>[3x]MTPE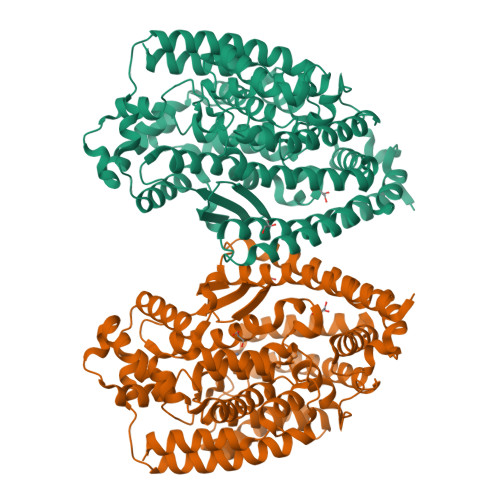AAYQNLLEFQRETAYLASLGALAAWDQRTMIPKKGHEHRARQMAALARLLHQRMTDPRIGEWLEKVEGSPLVQDPLSDAAVNVREWRQAYERARAIPERLAVELAQAESEAESFWEEARPRDDWRGFLPYLKRVYALTKEKAEVLFALPPAPGDPPYGELYDALLDGYEPGMRARELLPLFAELKEGLKGLLDRILGSGKRPDTSILHRPYPVEAQRRFALELLSACGYDLEAGRLDPTAHPFEIAIGPGDVRITTRYYEDFFNAGIFGTLHEMGHALYEQGLPKEHWGTPRGDAVSLGVHESQSRTWENLVGRSLGFWERFFPRAREVFASLGDVSLEDFHFAVNAVEPSLIRVEADEVTYNLHILVRLELELALFRGELSPEDLPEAWAEKYRDHLGVAPKDYKDGVMQDVHWAGGLFGYFPTYTLGNLYAAQFFQKAEAELGPLEPRFARGEFQPFLDWTRARIHAEGSRFRPRVLVERVTGEAPSARPFLAYLEKKYAALYG>[4x]MNLPTAQEVQGLMARAIELVDVGDIEAIVQMYADDATVEDPFGQPPIHG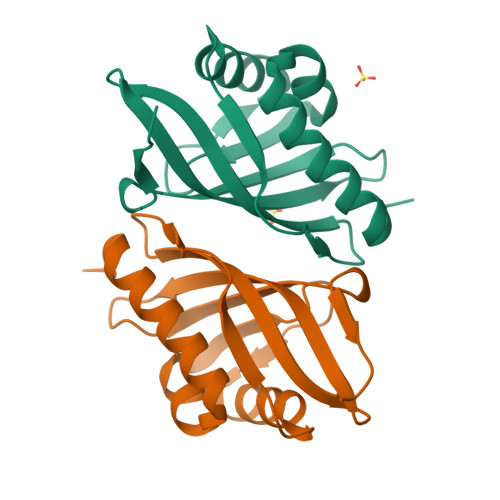REQIAAFYRQGLGGGKVRACLTGPVRASHNGCGAMPFRVEMVWNGQPCALDVIAVMRFDEHGRIQTMQAYWSEVNLSVREPQ> MSSQVEHPAGGYKKLFETVEELSSPLTAHVTGRIPLWLTGSLLRCGPGLFEVGSEPFYHLFDGQALLHKFDFKEGHVTYHRRFIRTDAYVRAMTEKRIVITEFGTCAFPDPCKNIFSRFFSYFRGVEVTDNALVNIYPVGEDYYACTETNFITKVNPETLETIKQVDLCNYVSVNGATAHPHIENDGTVYNIGNCFGKNFSIAYNIVKIPPLQADKEDPISKSEIVVQFPCSDRFKPSYVHSFGLTPNYIVFVETPVKINLFKFLSSWSLWGANYMDCFESNETMGVWLHIADKKRKKYINNKYRTSPFNLFHHINTYEDHEFLIVDLCCWKGFEFVYNYLYLANLRENWEEVKKNARKAPQPEVRRYVLPLNIDKADTGKNLVTLPNTTATAILCSDETIWLEPEVLFSGPRQAFEFPQI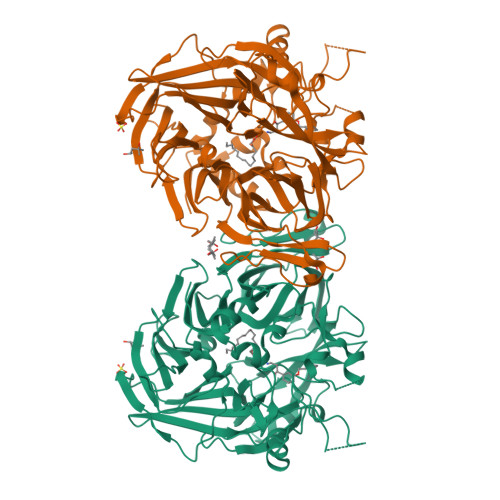NYQKYGGKPYTYAYGLGLNHFVPDRLCKLNVKTKETWVWQEPDSYPSEPIFVSHPDALEEDDGVVLSVVVSPGAGQKPAYLLILNAKDLSEVARAEVEINIPVTFHGLFKKS>[2x]GGHHWTYEGPHGQDHWPTSYPECGGDAQSPINIQTDSVIF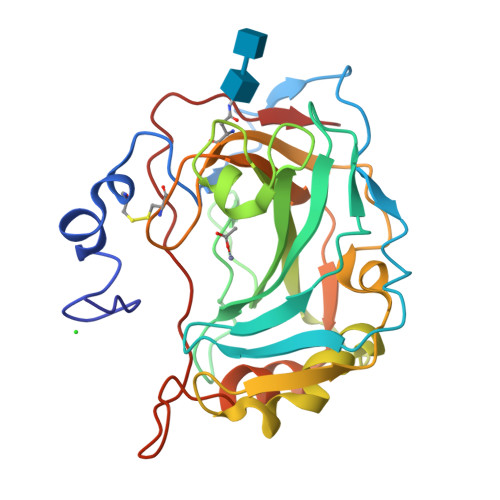DPDLPAVQPHGYDQLGTEPLDLHNNGHTVQLSLPPTLHLGGLPRKYTAAQLHLHWGQRGSLEGSEHHINSEATAAELHVVHYDSQSYSSLSEAAQKPQGLAVLGILIEVGETENPAYDHILSRLHEIRYKDQKTSVPPFSVRELFPQQLEQFFRYNGSLTTPPCYQSVLWTVFNRRAQISMGQLEKLQETLSSTEEDPSEPLVQNYRVPQPLNQRTIFASF>EQARPYAIPAGQLGDVLNRFAREAGITLSATPAQTGGYSSQGLRGSFTVQQGLARLLADTPLEAEDQGDGSFVLREAPAKDGDVLNMQAVEVFALGNNLGSTDGYLATHSQIATKTSKPLLETSQTVSVITREQIDDTASKTVQQAMRYTPGIFTGQVGASNRYDYVVMRGFADNSVDNIYLDGLKAMGDSGTFSSMQVDPYFLERIDVLKGPSSVLYGRSLPGGLVALTSKKPLYEDYRQITGSIGNMGQKEMGFDFSGPLDEEKRIAYRLIGLGKGSDTQFDHVKEERYAIAPTLAIDFSDDTTLTLQGYLQHDPNGGYHGGVPADGTLSHHNGRHISREFFDGEPSKDDFDRTQRMFGYQLEHRIDDVWSARQNFRYLDSDVDLSQVYAYGWSASEPNKLNRYFSGAREHLQAYIVDNMLQAEFATGAARHTLLTGLDYQRRRTVVDWRSGSASALDAFNPVYGDDAISYFPDDNHTRRLEQTGVYLQDLIDIDQWRFSLGLRQDWVSVTDKNRSTGSKADDDWEKFTGRIGALYLFDNGLAPYVSYSESFNPNAYSDASGTPLAPTEGKQWELGLKFQAPGSNSFYTASLFHITQENVASKEPQDNFYTSVGEVRSQGLELEAHTQLSDNLKLLGSYTYTDITYTKSLDGNQGHTPNQAPKHMASLWADYAFDAGPLSGLSIGGGARYVGETWADKENTLRVPDYTLVDARIGYDLGKLGLKGLDVSLNANNLLDKDYVASCYSLDFC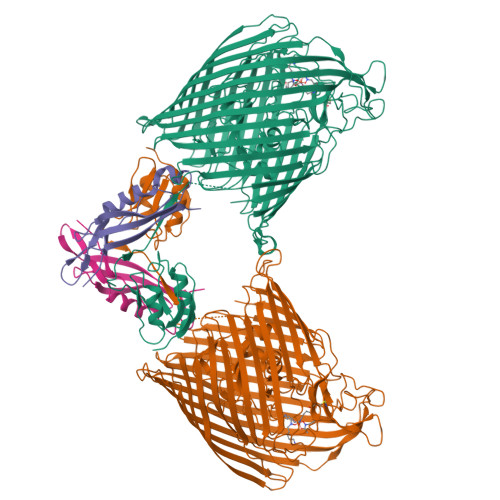YFGEKRNVTATVNYQF[2x];>[2x]DSDIKPLRMDPPVYPRMAQARGIEGRVKVLFTITSDGRIDDIQVLESVPSRMFDREVRQAMAKWRFEPRVSGGKIVARQATKMFFFKIEK>VARPKSEDKKQALLEAATQAIAQSGIAASTAVIARNAGVAEGTLFRYFATKDELINTLFLHLKQDLSQSMIMELDRSITDAKMMTRFIWNSYISWGLNHPARHRAIRQLAVSEKLTKETEQRADDMFPELRDLSHRSVLMVFMSDEYRAFGDGLFLALAETTMDFAARDPARAGEYIALGFEAMWRAL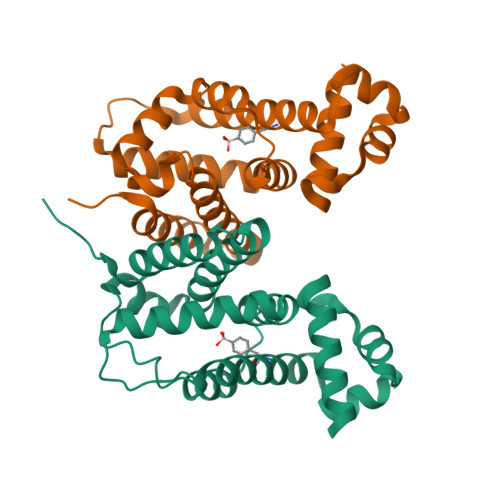TREEQAAWSHPQFEK[4x]~{N}-[3-[[3-[3-[3-[3-[(4-hydroxyphenyl)carbothioylamino]propanethioylamino]propanethioylamino]propylamino]-3-sulfanylidene-propyl]amino]-3-sulfanylidene-propyl]-4-oxidanyl-benzenecarbothioamide | C29 H38 N6 O2 S6 | 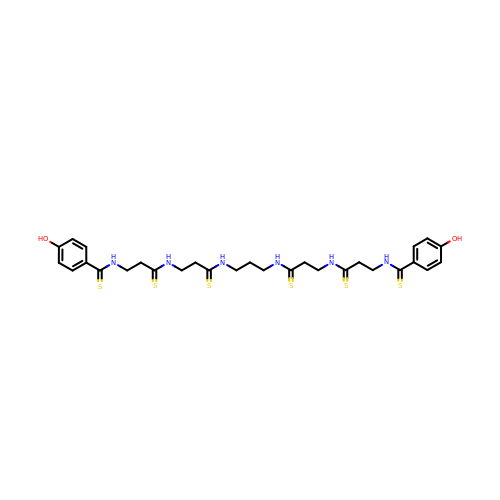UBZKZUDCUOZCCY-UHFFFAOYSA-N>MKNIGWMLRQRATVSPRLQAYVEPSTDVRMTYAQMNALANRCADVLTALGIAKGDRVALLMPNSVEFCCLFYGAAKLGAVAVPINTRLAAPEVSFILSDSGSKVVIYGAPSAPVIDAIRAQADPPGTVTDWIGADSLAERLRSAAADEPAVECGGDDNLFIMYTSGTTGHPKGVVHTHESVHSAASSWASTIDVRYRDRLLLPLPMFHVAALTTVIFSAMRGVTLISMPQFDATKVWSLIVEERVCIGGAVPAILNFMRQVPEFAE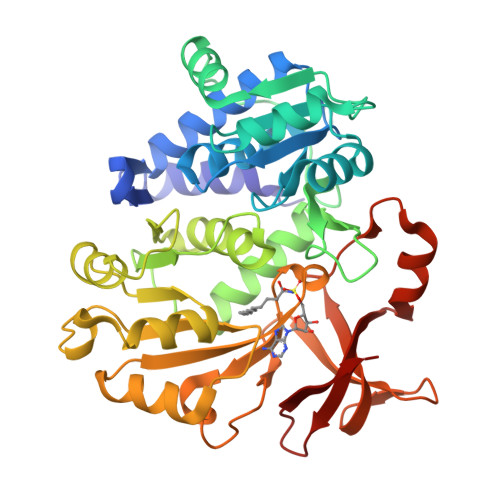LDAPDFRYFITGGAPMPEALIKIYAAKNIEVVQGYALTESCGGGTLLLSEDALRKAGSAGRATMFTDVAVRGDDGVIREHGEGEVVIKSDILLKEYWNRPEATRDAFDNGWFRTGDIGEIDDEGYLYIKDRL[2x]5-HYDROXYMETHYL URACIL | C5 H6 N2 O3 | 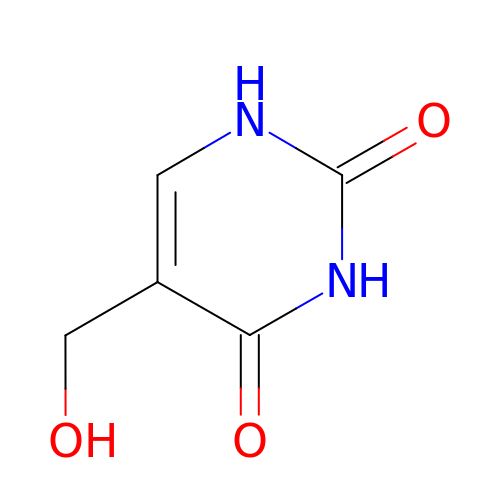JDBGXEHEIRGOBU-UHFFFAOYSA-N Saccharoymces cerevisiae Ess1 (Essential in yeast 1) is the founding member of the eukaryotic parvulin-class of peptidyl prolyl cis–trans isomerase (prolyl isomerase; PPIase). Ess1 and Pin1 are small modular proteins (~19.5 kDa) composed of two compact domains; an N-terminal Type-IV WW domain22 and C-terminal catalytic (PPIase) domain. Ess1 isomerizes the CTD of Rpb1, facilitating the recruitment of proteins needed for efficient transcription and RNA processing. Ess1 has a rigid linker between its WW and catalytic domains that enforces a distance constraint for bivalent interaction with the ends of long CTD substrates (≥4–5 heptad repeats).

S. cerevisiae Ess1 (henceforth called Ess1) was co-crystallized with a single heptad repeat (1R) phospho-Ser5 CTD peptide and the X-ray structure was determined at 2.4 Å resolution. The Ess1 N-terminal WW domain (residues 10–45) forms a three stranded anti-parallel β-sheet as described for Type IV WW-domains that recognize phospho-Ser-Pro motifs, and is highly similar to those in Pin1 and CaEss1, superimposing with an RMSD of 0.7 Å. A peak of positive electron density in the WW domain near W38 and Y27 was observed that we interpret as the position of proline 6 of the heptad repeat, as observed in the Pin1-CTD structure. The remainder of the CTD peptide was disordered and could not be modeled. The PPIase domain of Ess1 (aa 64–170) has a globular α/β-fold structure nearly identical to that of Pin1 and CaEss1, which superimposes with RMSDs of <0.7 and 0.6 Å, respectively. The entrance to the active site in Ess1 is formed by a large loop (aa 68–85) that includes basic residues K68, R73, R74, similar to those in Pin1 (K63, R68, R69) that interact with the phosphate group of pSer-Pro substrates. In the Ess1 structure, the basic loop is in the “closed” conformation as in CaEss127 and the original Pin1 structure, rather than in an “open” conformation seen in a later Pin1 structure. Key catalytic site residues identified in Pin1 (including H59, C113, H157, S115, Q131, F134)28,35–38 are conserved in Ess1 (H64, C120, H164, S122, Q138, F141) and located in analogous positions. Finally, in the Ess1 structure, the WW is even further removed and occupies a space on the opposite side from the PPIase domain α1-helix, generating an elongated structure. In contrast, the linker regions in Ess1 (K46-R59) and CaEss1 (K43-Q67) are highly ordered and contain a solvent-exposed, amphipathic α-helix (colored in magenta).

>MPSDVASSTGLPTPWTVRYSKSKKREYFFNPETKHSQWEEPEGTNKDQLHKHLRDHPVRVRCLHILIKHKDSRRPASHRSENITISKQDATDELKTLITRLDDDSKTNSFEALAKERSDCSSYKRGGDLGWFGRGEMQPSFEDAAFQLKVGEVSDIVESGSGVHVIKRVG[2x]(2R)-2-methyl-2-[[2-(1H-pyrrolo[2,3-b]pyridin-3-yl)pyrimidin-4-yl]amino]-N-[2,2,2-tris(fluoranyl)ethyl]butanamide | C18 H19 F3 N6 O | 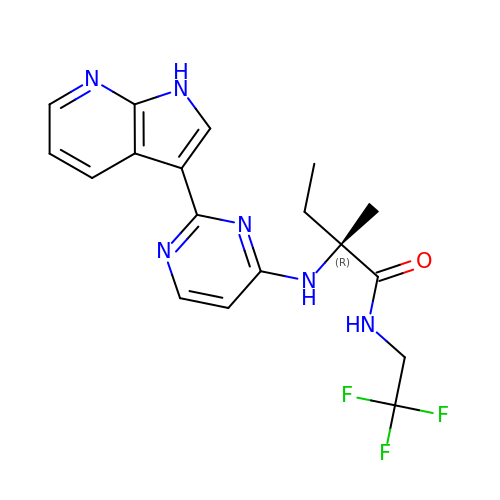ASUGUQWIHMTFJL-QGZVFWFLSA-N> MSHEGLSPIPGEGTGIQLSAGQILKFYNVPIAEIIVEYDPSNVSGVSSNVKLKGTIHPLFEVPSQISIENFQPTENYLIYSGFGTSLPQ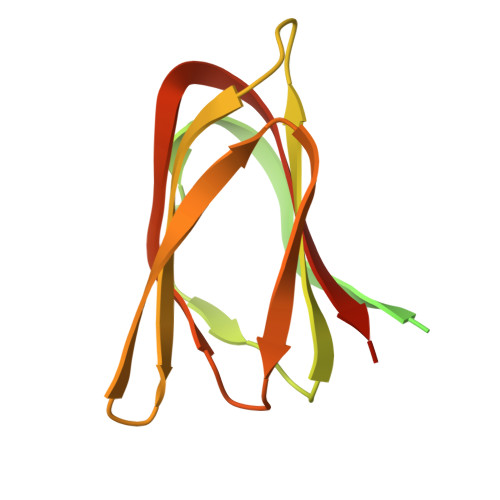TYTIPANGYLIISITNTSTGNIGQITLTIGSTTMTFNLQTGENKIPVIAGTQITNMTLTSSSAILIYEEVIHHHHHH> MRHISPEELIALHDANI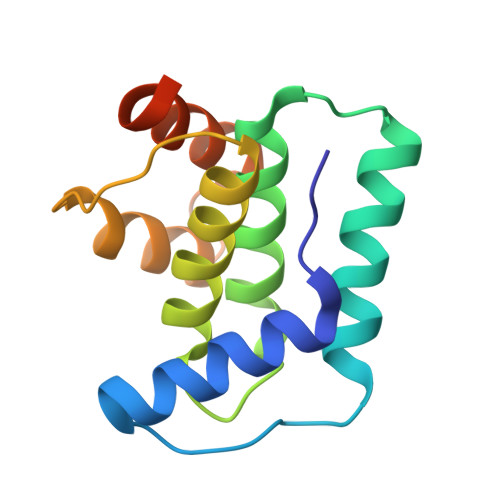SRYGGLPGMSDPGRAEAIIGRVQARVAYEEITDLFEVSATYLVATARGYIFNDANKRTALNSALLFLRRNGVQVFDSPELADLTVGAATGEISVSSVADTLRRLYGSADPLEHHHHHH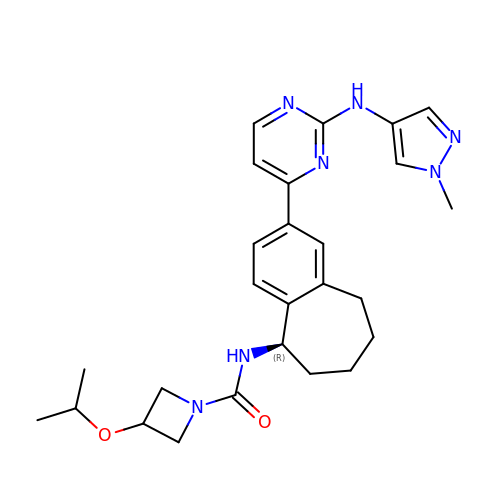~{N}-[(5~{R})-2-[2-[(1-methylpyrazol-4-yl)amino]pyrimidin-4-yl]-6,7,8,9-tetrahydro-5~{H}-benzo[7]annulen-5-yl]-3-propan-2-yloxy-azetidine-1-carboxamide | C26 H33 N7 O2 | HYNHKNQQFCVJGQ-XMMPIXPASA-N> VPSPYLLSDKEVREIVQQSLSVGNFAARLLVRLFPELFTAENLRLQYN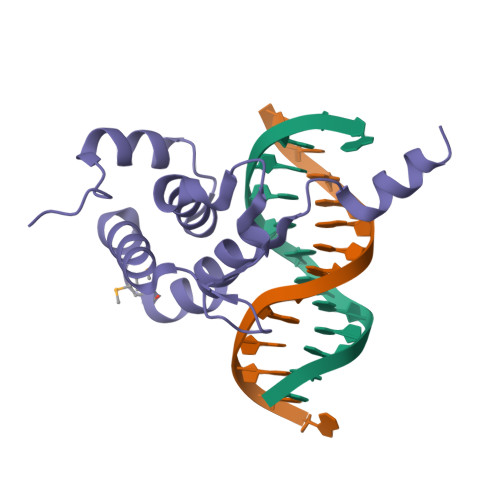HSGACNKKQLDPTRLRLIRHYVEAVYPVEKMEEVWHYECIPSIDERCRRPNRKKCDILKKAKK> MMEQVCDVFDIYAICACCKVESKNEGKKNEVFNNYTFRGLGNKGVLPWKCNSLDMKYFRAVTTYVNESK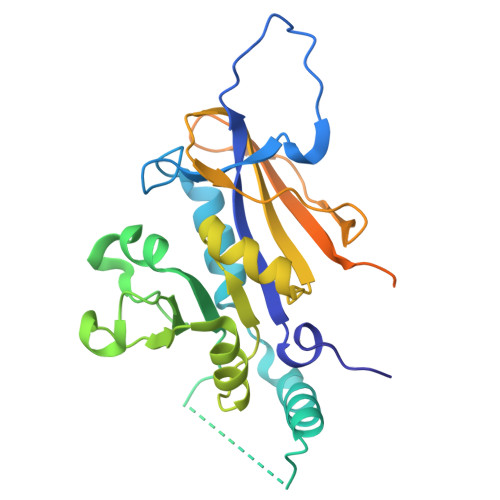YEKLKYKRCKYLNKETVDNVNDMPNSKKLQNVVVMGRTNWESIPKKFKPLSNRINVILSRTLKKEDFDEDVYIINKVEDLIVLLGKLNYYKCFIIGGSVVYQEFLEKKLIKKIYFTRINSTYECDVFFPEINENEYQIISVSDVYTSNNTTLDFIIYKKTNNKMLNEQNCIKGEEKNNDMPLKNDDKDTCHMKKLTEFYKNVDKYKINYEN TRIPHOSPHATE | H5 O10 P3 | 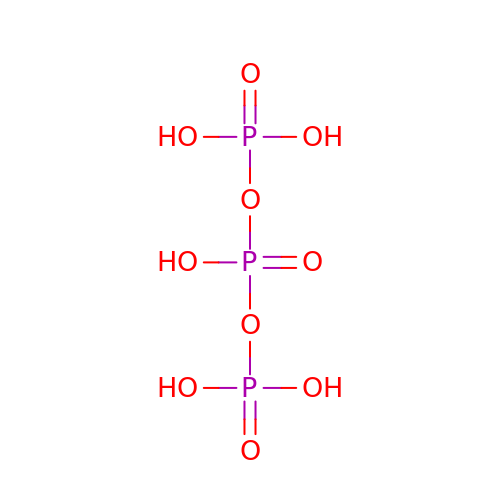UNXRWKVEANCORM-UHFFFAOYSA-N> MAYSDVDAILADGKQAVAVKHGGGLVVVGELGAQVLAAKDVSELPDGVGGTAPGAATTTTAGV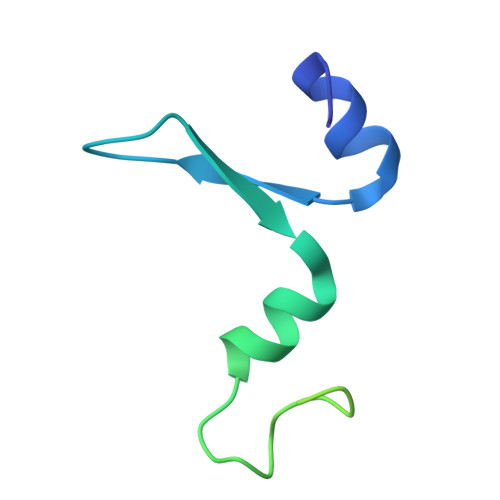VKQSTTQAASVATDVAGVVTDLNALITKLKAAGIMA>MSQTDARRSGRFLRTVEWLGNMLPHPVTLFIIFIVLLLIASAVGAYFGLSVPDPRPVGAKGRADDGLIHVVSLLDADGLIKILTHTVKNFTGFAPLGTVLVSLLGVGIAEKSGLISALMRLLLTKSPRKLTTFMVVFTGILSNTASELGYVVLIPLSAVIFHSLGRHPLAGLAAAFAGVSGGYSANLFLGTIDPLLAGITQQAAQIIHPDYVVGPEANWFFMAASTFVIALIGYFVTEKIVEPQLGPYQSDLSQEEKDIRHSNEITPLEYKGLIWAGVVFIALSALLAWSIVPADGILRHPETGLVAGSPFLKSIVVFIFLLFALPGIVYGRITRSLRGEREVVNAMAESMSTLGLYLVIIFFAAQFVAFFNWTNIGQYIAVKGAVFLKEVGLAGSVLFIGFILICAFINLMIGSASAQWAVTAPIFVPMLMLAGYAPEVIQAAYRIGDSVTNIITPMMSYFGLIMATVMKYKKDA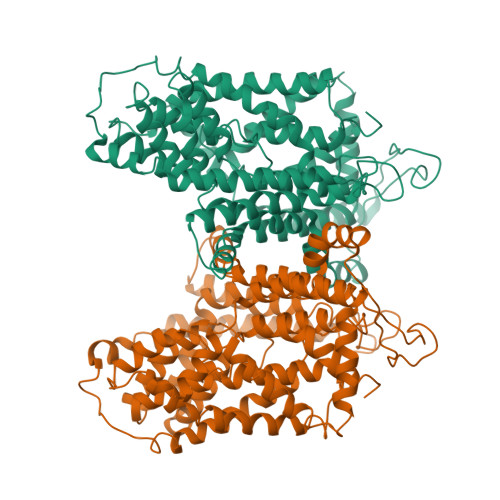GVGTLISMMLPYSAFFLIAWIALFCIWVFVLGLPVGPGAPTLYPAP[2x]> MTITLIEPVQQRTGIYPSSDLKVEDGYPSSDTFQIIQTQDGRGAGVRVLKTFARGRRMARVSGQITAFCRLHTLQINAHTHLYDPHFSGLLLHSCVPNVRLDMAGFELWSLRDIAAGEMLTMDYASTEDVLMRQFECHCGAPNCRRWITGAKELPNDIGQALLAGLRAAALALEHHHHHH

BurB, a SET (Suppressor of variegation, Enhancer of zeste and Trithorax) domain-containing enzyme identified from Burkholderia thailandensis, initiates DMSP synthesis by methylating methionine (Met) to S-methyl-methionine (SMM), with S-adenosyl methionine (SAM) as a methyl donor. BurB is a S-adenosyl methionine (SAM)-dependent Met S-methyltransferase containing a SET (Suppressor of variegation, Enhancer of zeste and Trithorax) domain, and belongs to the class V of the methyltransferase superfamilies. The SET domain proteins are well known for their roles in methylating histone lysines in eukaryotes, and BurB represents a new member of the SET domain proteins. Each BurB monomer consists of eight β-sheets and four α-helices.

The crystals of BurB-SMM-SAM complex belong to the I222 space group, and there is only one BurB molecule in an asymmetric unit. In the BurB-SMM-SAM complex, the SMM molecule is located in the same position as Met in the BurB-Met complex. In addition to the SMM molecule, the SAM molecule was also clearly observed in the BurB-SMM-SAM complex structure. Residues His93 and His138 form hydrogen bonds with the SAM adenine ring. The side chain of Arg133 interacts with the ribose ring. The amino and carboxyl groups of SAM contact with residues Arg42, Ala44, and His72 via hydrogen bonds. In the BurB-Met complex, the Met molecule is accessible to the surface, suggesting that BurB possesses an open conformation. After the SAM molecule enters into the substrate-binding pocket, the loop (Gln37-Ala44) generates a conformational change (Fig. 5C through E) and participates in binding SAM via the residues Arg42 and Ala44. Structural analysis of the BurB-SMM-SAM complex indicated that either residue Tyr124 or Ser88, which are located between the SMM molecule and the SAM molecule, may act as the catalytic residue. After SAM enters the substrate binding pocket, BurB generates a conformational change to form the closed conformation, which brings the sulfur atom of Met in close proximity to the SAM methyl group and allows the nucleophilic attack on the methyl group.> GAMENKKARKSKCIIMSKSIQGLPIKWEEYAADEVVLLVPTSHTDGSM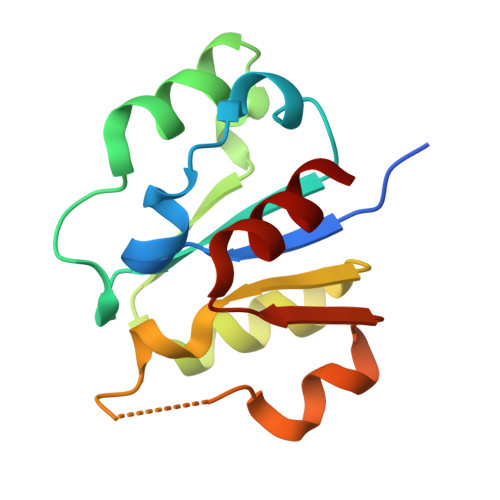KQAIGDAFRKTKNEHKIIYCDSMDGLWSCVRRLGKFQCILNSRDFTSSGGSDAAVVPEDIGRFVKFVVDSDVEDVLIDTLCN>[2x]VGVNPLPAPREISWGSSGPKSIAGELQLRTDSDSADGIVADAWNRAWETIVALRWVPAATEAPISSFEPFPTPTAGAS;>[2x]ASNSLQYVNVQVKDIEADLQHGVDESYTLDVEEDSDTITINAETVWGALHAFTTLQQLVISDGHGGLIIEEPVNIKDSPLYPYRGIMLDTGRNFVSLPKIFEQLEGMSLSKLNVLHWHIDDAQSWPIWVDVYPEMVKDAYSPHEIYSRNDVRNIVNYARARGIRVIPEIDMPSHSSSGWKQVDPEMVTCTDSWWSNDDWPLHTAVEPNPGQLDIIYNKTYEVVGNVYKELSDIFPDHWFHVGGDEIQPNCFNFSTHVTKWFAEDPSRTYHDLAQYWVDHAVPIFQNYSQERRLVMWEDIALSADNAHDVPKNIVMQSWNNGLEYISNLTARGYDVIVSSSDFLYLDCGHGGF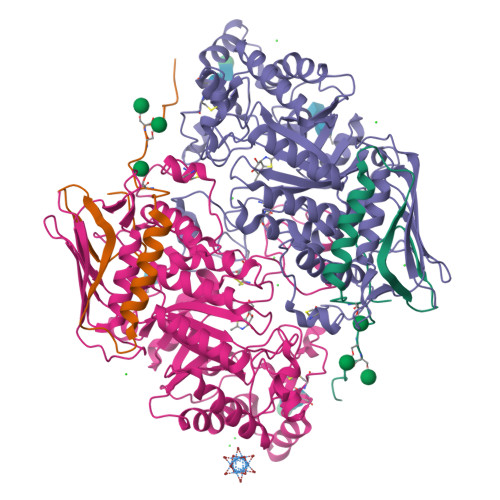VTNDPRYNVMANPDANTPNFNYGGNGGSWCAPYKTWQRIYDYDFTLNLTETQAKHIIGATAPLWGEQVDDINVSSMFWPRAAALAELVWSGNRDANGNKRTTEMTQRILNFREYLVANGVQAQALVPKYCLQHPHACDLYRNQAAIQ>MGSSHHHHHHSSGRENLYFQGHMSKFTIHTIETAPERVKETLRTVKKDNGGYIPNLIGLLANAPTALETYRTVGEINRRNSLTPTEREVVQITAAVTNGCAFCVAGHTAFSIKQIQMAPDLLEALRNATPIDDDPKLDTLAKFTIAVINTKGRVGDEAFA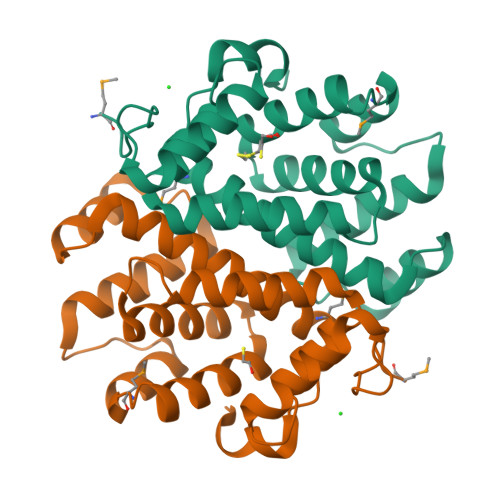DFLEVGYTPENALDVVLGVSLASLCNYANNMADTPINPELQQYVKGS[6x]ELLIPTICINE | C17 H15 N2 | 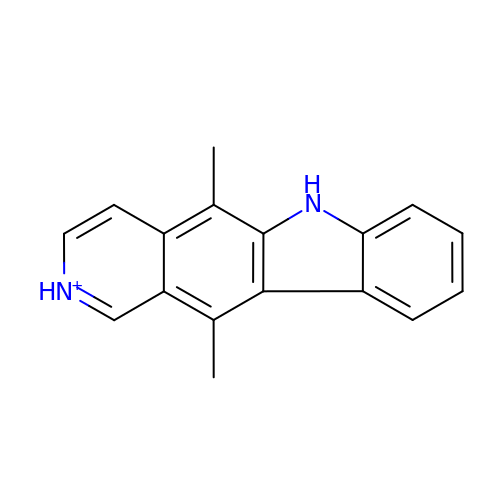CTSPAMFJBXKSOY-UHFFFAOYSA-O>MHHHHHHSSENLYFQGHMASMRIPEDVRKDIPLTNEVIYFDNTATSLTPKPVVEAMDEYYLKYRANVHRGVHRLSQMATHKYEESRKIVADFIGAKFEEIVFTKNTSESLNLVALGLGHIFKRGDKIVTTPYEHHSDLLPWQRLATKLGLKLEFIEGDDEGNLDLSDAEKKIKGAKLVAVQHVSNALGVIHEVEELGKIAKDEGAIFVVDAAQSAGHMEVNVKKLHADFLAFSGHKGPMGPTGIGVLYIREEFFDTFEPPLIGGGTIEDVSLDGYKLTEPPERFEAGTPNIGGAIGLAAGIRYIERIGLGRIERQEHKLVKRTTEGLDELEVPWYGPRNLKKHAGVVSFNVPGLHPHDVAAI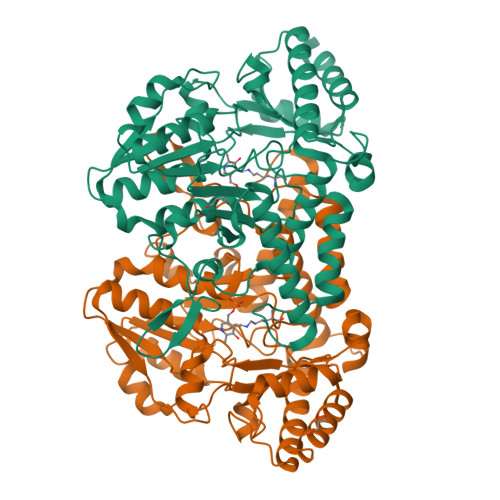LDDHSIMVRSGHHCALPVMKKLGINGTVRASFHVYNSLEEVETFLGVMEELVKGLKT[2x]> SGDPIPDMSKFATGITPFEFENMAESTGMYLRIRSLLKNSPRNQQK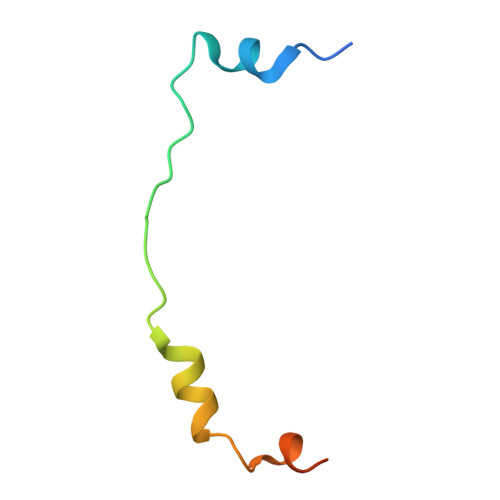NKKASE(1R,3S,5Z)-5-[(2E)-2-[(1R,3aS,7aR)-1-[(2R,3S)-3-(2-hydroxyethyl)heptan-2-yl]-7a-methyl-2,3,3a,5,6,7-hexahydro-1H-inden-4-ylidene]ethylidene]-4-methylidene-cyclohexane-1,3-diol 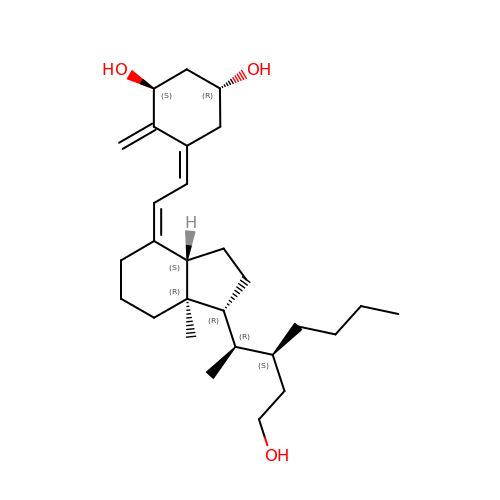| C28 H46 O3 | MBUIFNPNESWHQQ-LGKYDQOKSA-N6-[(3-aminopropyl)amino]-N-hydroxyhexanamide | C9 H21 N3 O2 | 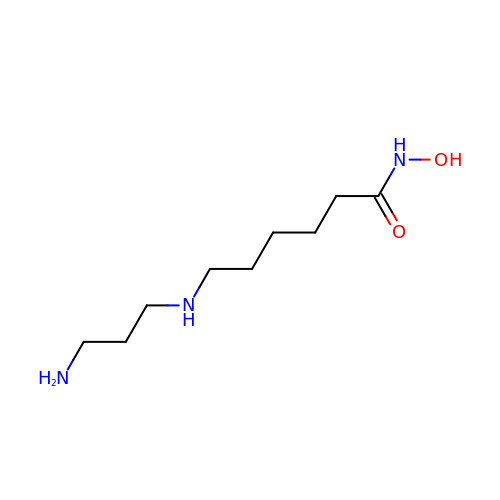BREASWSBOVLQOH-UHFFFAOYSA-N> GHMQTSHKKVRFDEGSYTNFIYDNKSYFVTDKEIPQENVNNSKVKFYKLLIVDMKSEKLLSSSNKNSVTLVLNNIYEASDKSLCMGINDRYYKILPESDKGAVKALRLQNFDVTSDISDDNFVIDKNDSRKIDYMGNIYSISDTTVSDEELGEYQDVLAEVRV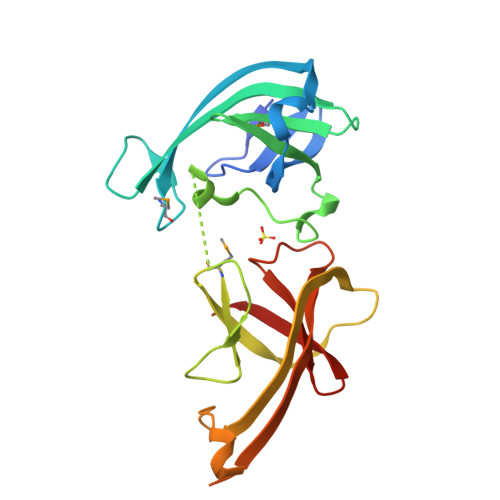FDSVSGKSIPRSEWGRIDKDGSNSKQSRTEWDYGEIHSIRGKSLTEAFAVEINDDFKLATKVGNLE> VFPSSVFVPDEWEVSREKITLLRELGQGSFGMVYEGNARDIIKGEAETRVAVKT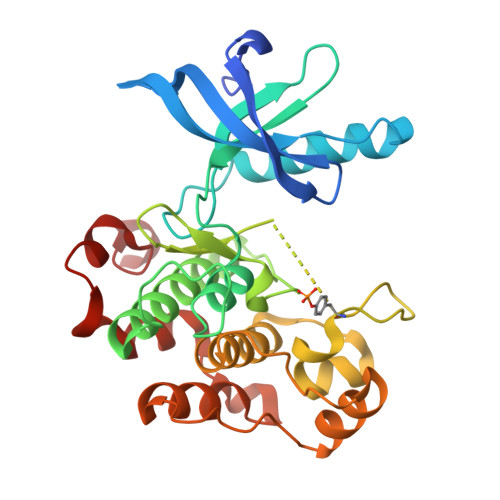VNESASLRERIEFLNEASVMKGFTCHHVVRLLGVVSKGQPTLVVMELMAHGDLKSYLRSLRPEAENNPGRPPPTLQEMIQMAAEIADGMAYLNAKKFVHRDLAARNCMVAHDFTVKIGDFGMTRDIYETDYYRKGGKGLLPVRWMAPESLKDGVFTTSSDMWSFGVVLWEITSLAEQPYQGLSNEQVLKFVMDGGYLDQPDNCPERVTDLMRMCWQFNPKMRPTFLEIVNLLKDDLHPSFPEVSFFHSEENK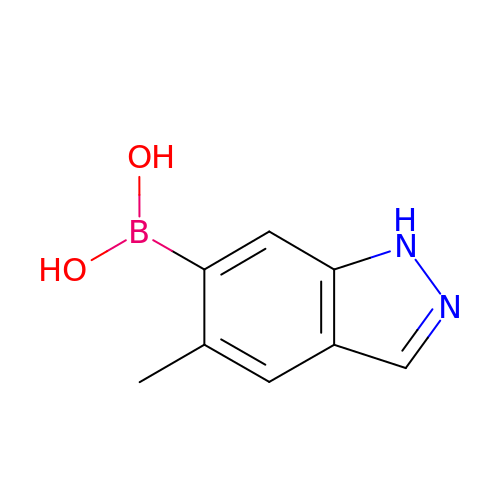(5-methyl-1H-indazol-6-yl)boronic acid | C8 H9 B N2 O2 | FVSYCXICBAFOGW-UHFFFAOYSA-N N~2~-[(4-fluoro-3-methylphenyl)sulfonyl]-N-hydroxy-N~2~-methyl-D-alaninamide 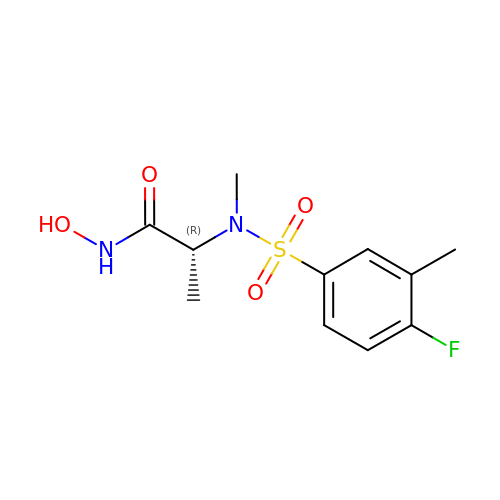| C11 H15 F N2 O4 S | WVQNSSTZICUBDI-MRVPVSSYSA-N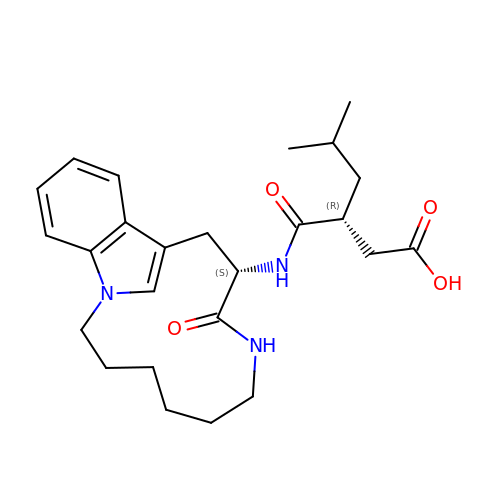5-METHYL-3-(9-OXO-1,8-DIAZA-TRICYCLO[10.6.1.013,18]NONADECA-12(19),13,15,17-TETRAEN-10-YLCARBAMOYL)-HEXANOIC ACID | C25 H35 N3 O4 | AKWKBACKRMYPRV-NQIIRXRSSA-N> MASDMEEKFREAFILF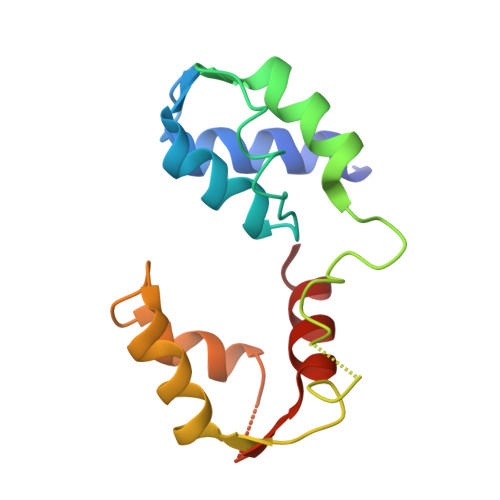SSCSDHIEMYKFFELMNSFGIILTNDEKAALPNDINMDYWLNFAKKHYNYEQPFKHINNVNEQNTNVQIKIDNFLGIMKALDTRLTESDLNILLQITNPENKSTLNLKTVSQKLTESI>[2x]QEVEFDIPPQALGSALQEFGRQADIQVLYRPEEVRNKRSSAIKGKLEPNQAITELLRGTGASVDFQGNAITISVAEAADSSVDLGATMITSNQLGTITEDSGSYTPGTIATATRLVLTPRETPQSITVVTRQNMDDFGLNNIDDVMRHTPGITVSAYDTDRNNYYARGFSINNFQYDGIPSTARNVGYSAGNTLSDMAIYDRVEVLKGATGLLTGAGSLGATINLIRKKPTHEFKGHVELGAGSWDNYRSELDVSGPLTES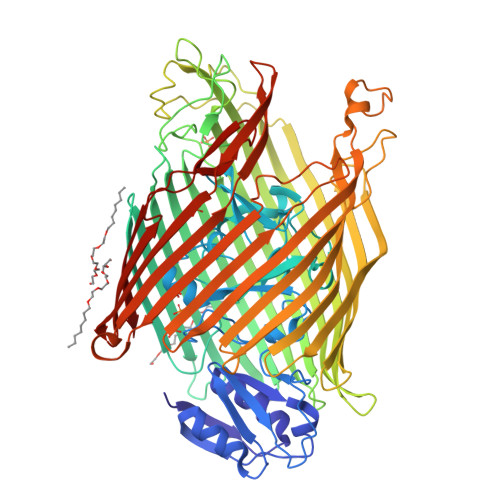GNVRGRAVAAYQDKHSFMDHYERKTSVYYGILEFDLNPDTMLTVGADYQDNDPKGSGWSGSFPLFDSQGNRNDVSRSFNNGAKWSSWEQYTRTVFANLEHNFANGWVGKVQLDHKINGYHAPLGAIMGDWPAPDNSAKIVAQKYTGETKSNSLDIYLTGPFQFLGREHELVVGTSASFSHWEGKSYWNLRNYDNTTDDFINWDGDIGKPDWGTPSQYIDDKTRQLGSYMTARFNVTDDLNLFLGGRVVDYRVTGLNPTIRESGRFIPYVGAVYDLNDTYSVYASYTDIFMPQDSWYRDSSNKLLEPDEGQNYEIGIKGEYLDGRLNTSLAYFEIHEENRAEEDALYNSKPTNPAITYAYKGIKAKTKGYEAEISGELAPGWQVQAGYTHKIIRDDSGKKVSTWEPQDQLSLYTSYKFKGALDKLTVGGGARWQGKSWQMVYNNPRSRWEKFSQEDYWLVDLMARYQITDKLSASVNVNNVFDKTYYTNIGFYTSASYGDPRNLMFSTRWDF;> SAAADAS>MFELVDNIAQTAVIKVIGVGGGGGNAVNHMAKNNVEGVEFICANTDAQALKNIAARTVLQLGPGVTKGLGAGANPEVGRQAALEDRERISEVLEGADMVFITTGMGGGTGTGAAPIIAEVAKEMGILTVAVVTRPFPFEGRKRMQIADEGIRALAESVDSLITIPNEKLLTILGKDASLLAAFAKADDVLAGAVRGISDIIKRPGMINVDFADVKTVMSEMGMAMMGTGCASGPNRAREATEAAIRNPLLEDVNLQGARGILVNITAGPDLSLGEYSDVGNIIEQFASEHATVKVGTVIDADMRDELHVTVVATGLGARL[2x];>PAAFSELSLSGLPGHCLTLLAPILRELSEEQDARWLTLIAPPASLTHEWLRR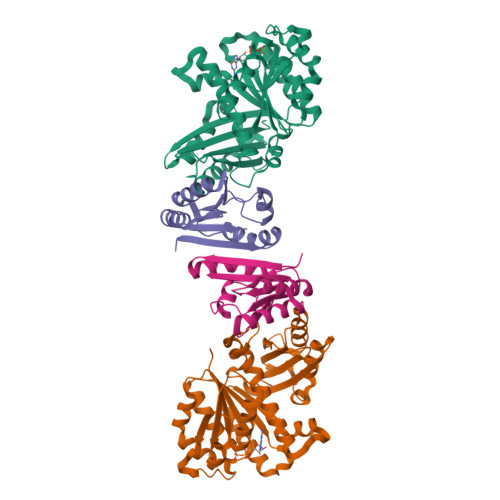AGLNRERILLLQAKDNAAALALSCEALRLGRSHTVVSWLEPLSRAARKQLSRAAQLGQAQSLNIRLG[2x]>MEASRRDFISIGIGALGAVGGLGALYALVRVMLEPSEIAALGAKTEIDVSKIQPMQVRVTSWKGKTLFAIRLPKDFKPEGYTLKKGALNSKGTTNYEILKGHDVFALVGVCTHLGCIPLWKPQGEGGINKPVFHCPCHGGLYTPYGDVIGGPPPRPLFIPPQKLEGNKLIVGVEGFVKELI[2x];>[2x]MGLIEKIVDWIDERAHVREIYRTQMVEYKVAKNLTFPYVFGILALVTFAIQIISGMVLILYYKPSIADAFDSATYSIMGEIPFGWLFRHIHATGANFFMAIVYLHMFTGIYYNAYKRPRELVWIVGWLIYFVLILTALSGYLLPWGQLSYWGFIVTTEIPGSLADAPILKPIFKAIAETIVLWMKGGYVVTDVTLGRVFGSHVLIYPLILLALVGIHLYLVRAAGISNPEGIEYDKKKNPDKFVPFHPYMTLKEGAYVMWYLAVFFFFVFFHISHFLPPENFEPANPLKTPAHIAPEWYLLGYYEVFRSIPSKFWGFVAFNALLLLLLLLPFLDFSPLKSARRRPLFFVMFVIFMISSMALTILGTMPPTPQNAKLGLIFAALVFAFFISLPIISFIEYGWYKAKGGQQE;>[2x]MNTWGLIKTIFFAGSTLVFFFLLWFYNPFKHVEHYEVDEEVKAIIDNPWKKTESGKTIAEEGRELFIASCSSCHSLRYDGIYIMSVAANPKWKNIEKTSGRPVYRFGT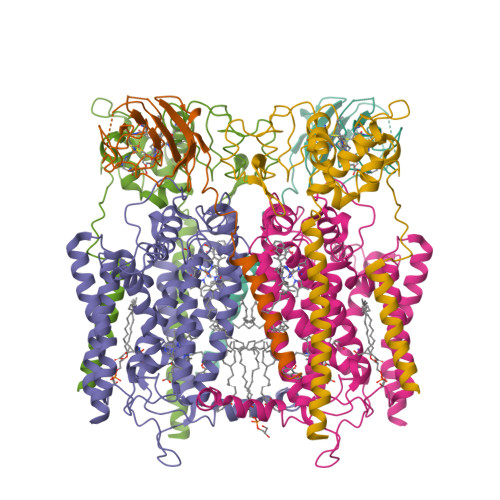LYKDRFFVPKDVYEAFAHDDIQGLKASLGQVPPDLSSMYLARGEGYLYQFILNPQKVLPGTTMPQLFNPQFDPQAKEKVAKIVAYMKSVNTPPPKESAKRTVMGVIVIAYFIVMGLLLWKYRENLLKRLGYH>ISTLHHQTMPSDLTQDEFTQLSQSIAEFHTYQLGNGRCSSLLAQRIHAPPETVWSVVRRFDRPQIYKHFIKSCNVSEDFEMRVGCTRDVNVISGLPANTSRERLDLLDDDRRVTGFSITGGEHRLRNYKSVTTVHRFEKEEEEERIWTVVLESYVVDVPEGNSEEDTRLFADTVIR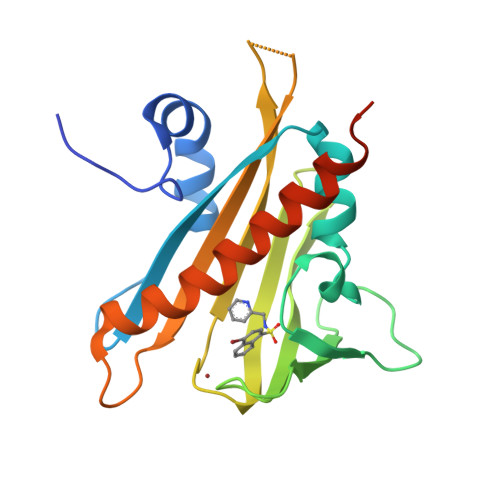LNLQKLASITEAMNRNNNNNNSSQVR[2x]>[2x]RRYTLNATALGLGGAATRQLTFQTSSPAHLTMPYVMPGDGEVVGVGEPVAIRFDENIADRGAAEKAIKITTNPPVEGAFYWLNNREVRWRPEHFWKPGTAVDVAVNTYGVDLGEGMFGEDNVQTHFTIGDEVIATADDNTKILTVRVNGEVVKSMPTSMGKDSTPTANGIYIVGSRYKHIIMDSSTYGVPVNSPNGYRTDVDWATQISYSGVFVHSAPWSVGAQGHTNTSHGALNVSPSNAQWFYDHV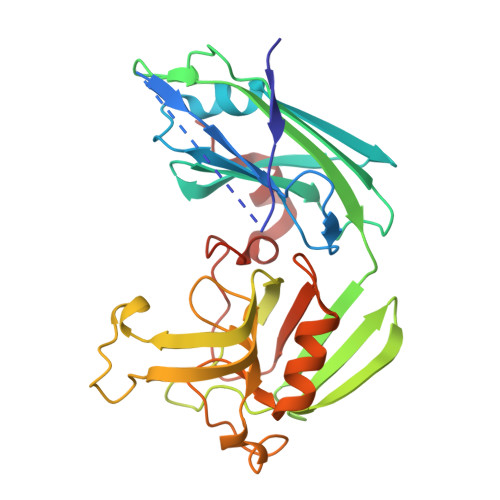KRGDIVEVVNTVGGTLPGIDGLGDWNIPWDQWRAGNAKA> AEALSPEQAAHYLRYVKEAKEATK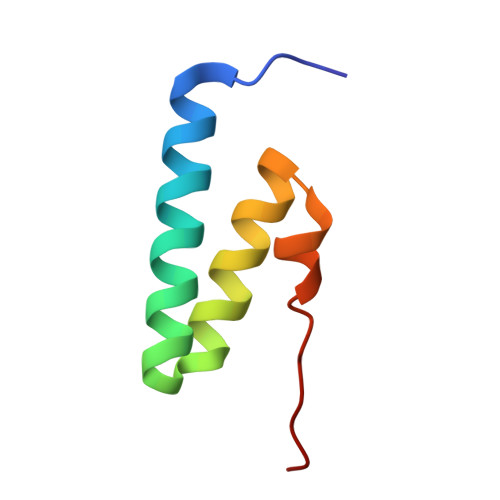NGDLEEAFKLFNLAKDIFPNEKVLSRIQKIQEA(R)-1-(4-(4-(HYDROXYMETHYL)-1,3,2-DIOXABOROLAN-2-YL)PHENETHYL)GUANIDINE 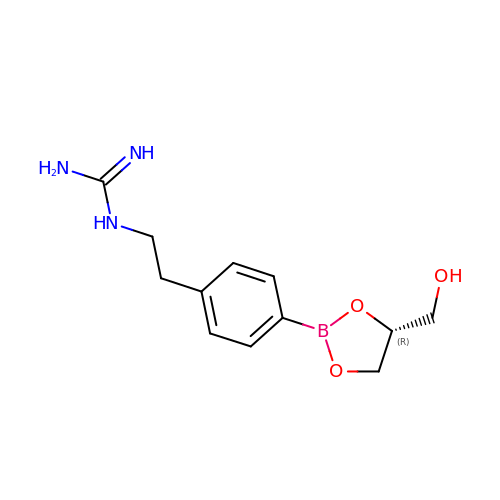| C12 H18 B N3 O3 | ZYCNKSJMJFKCBX-LLVKDONJSA-N>ATTGTQGYTVVKNDWKKAVKQLQDGLKDNSIGKITVSFNDGVVGEVAPKSANKKADRDAAAEKLYNLVNTQLDKLGDGDYVDFSVDYNLENKIITNQADAEAIVTKLNSLNEKTLIDIATKDTFGMVSKTQDSEGKNVAATKALKVKDVATFGLKSGGSEDTGYVVEMKAGAVEDKYGKVGDSTAGIAINLPSTGLEYAGKGTTIDFNKTLKVDVTGGSTPSAVAVSGFVTKDDTDLAKSGTINVRVINAKEESIDIDASSYTSAENLAKRYVFDPDEISEAYKAIVALQNDGIESNLVQLVNGKYQVIFYPEGKRLE[2x];>NDTIASQDTPAKVVIKANKLKDLKDYVDDLKTYNNTYSNVVTVAGEDRIETAIELSSKYYNSDDKNAITDKAVNDIVLVGSTSIVDGLVASPLASEKTAPLLLTSKDKLDSSVKSEIKRVMNLKSDTGINTSKKVYLAGGVNSISKDVENELKNMGLKVTRLSGEDRYETSLAIADEIGLDNDKAFVVGGTGLADAMSIAPVASQLKDGDATPIVVVDGKAKEISDDAKSFLGTSDVDIIGGKNSVSKEIEESIDSATGKTPDRISGDDRQATNAEVLKEDDYFTDGEVVNYFVAKDGSTKEDQLVDALAAAPIAGRFKESPAPIILATDTLSSDQNVAVSKAVPKDGGTNLVQVGKGIASSVINKMKD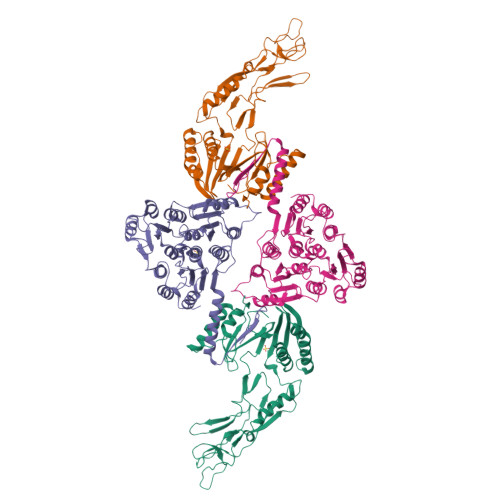LLDM[2x]> SATRANKDIFTLFDKKGQGAIAKDSLGDYLRAIGYNPTNQLVQDIINADSSLRDASSLTLDQITGLIEVNEKELDATTKAKTEDFVKAFQVFDKESTGKVSVGDLRYMLTGLGEKLTDAEVDELLKGVEVDSNGEIDYK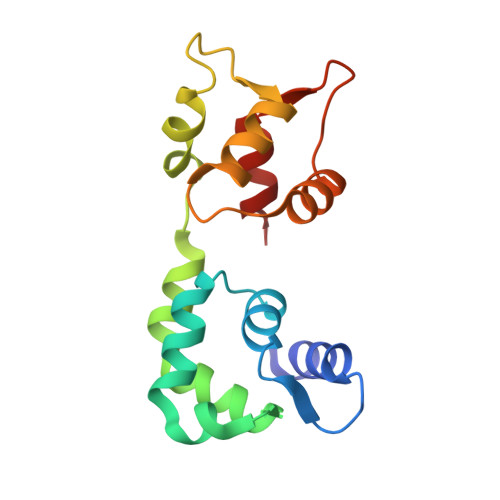KFIEDVLRQ>CGCGNAT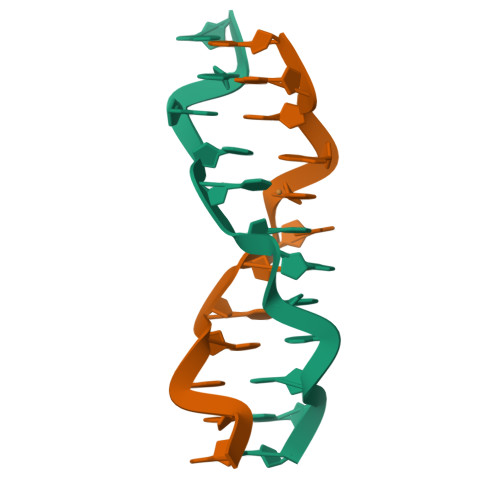NCGCG[2x]>[2x]MTAQISPTVVDAVVIGAGFGGIYAVHKLHNEQGLTVVGFDKADGPGGTWYWNRYPGALSDTESHLYRFSFD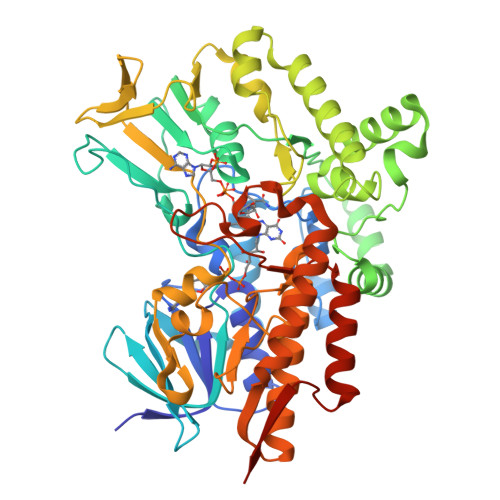RDLLQDGTWKTTYITQPEILEYLESVVDRFDLRRHFRFGTEVTSAIYLEDENLWEVSTDKGEVYRAKYVVNAVGLLSAINFPDLPGLDTFEGETIHTAAWPEGKNLAGKRVGVIGTGSTGQQVITALAPEVEHLTVFVRTPQYSVPVGNRPVTKEQIDAIKADYDGIWDSVKKSAVAFGFEESTLPAMSVSEEERNRIFQEAWDHGGGFRFMFGTFGDIATDEAANEAAASFIRSKIAEIIEDPETARKLMPTGLYAKRPLCDNGYYEVYNRPNVEAVAIKENPIREVTAKGVVTEDGVLHELDVLVFATGFDAVDGNYRRIEIRGRNGLHINDHWDGQPTSYLGVTTANFPNWFMVLGPNGPFTNLPPSIETQVEWISDTVAYAERNEIRAIEPTPEAEEEWTQTCTDIANATLFTRGDSWIFGANVPGKKPSVLFYLGGLGNYRNVLAGVVADSYRGFELKSAVPVTALEHHHHHH> GPLGSMS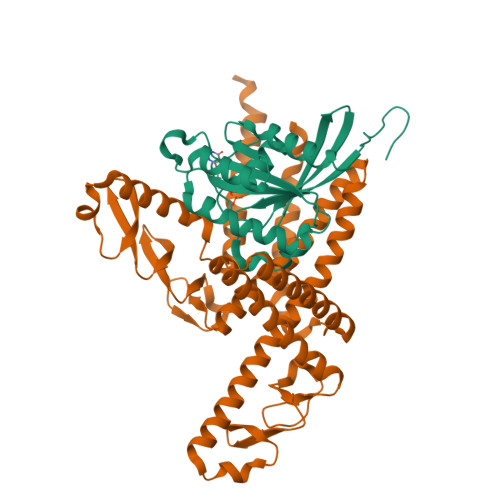SMNPEYDYLFKLLLIGDSGVGKNCLLLRFADDTYTESYISTIGVDFKIRTIELDGKTIKLQIWDTAGQERFRTITSSYYRGAHGIIVVYDVTDQESFNNVKQWLQEIDRYASENVNKLLVGNKCDLTTKKVVDYTTAKEFADSLGIPFLETSAKNATNVEQSFMTMAAEIKKRM;> KKLDKLERQGKDLEDKYKTYEENLEGFEKLLTDSEELSLSEINEKMKAFSKDSEKLTQLMEKHKGDEKTVQSLQREHHDIKAKLANLQVLHDAHTGKKSYVNEKGNPVSSLKDAHLAINKDQEVVEHKGQFYLLQKGQWDAIKNDPAALEKAQKDYSQSKHDLATIKMEALIHKLSLEMEKQLETINDLIMSTDPKENEEATKLLHKHNGLNLKLANLQDMLAVHRKEKSFFNEKGEKVTSLNDAHYVIGKDQQLFNLGGKFYPIHKEQKILEKDGKFYLLKQGEDWESIKDSPEKQKKAEHDFHKLQYETPMTVKKLVHHNKGLETTIHKERIEELEHHHHHH>[2x]PYTVVYFPVRGRCAALRMLLADQGQSWKEEVVTVETWQEGSLKASCLYGQLPKFQDGDLTLYQSNTILRHLGRTLGLYGKDQQEAALVDMVNDGVE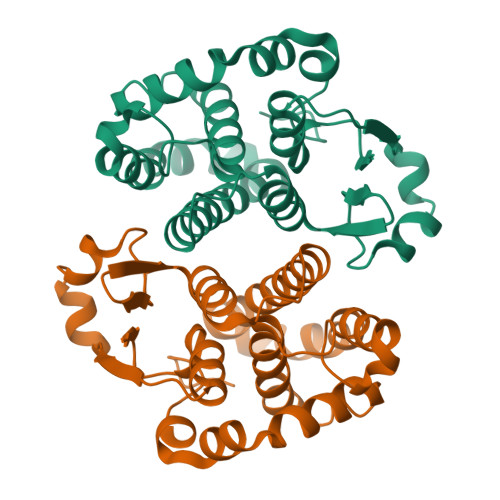DLRCKYISLIYTNYEAGKDDYVKALPGQLKPFETLLSQNQGGKTFIVGDQIAFADYNLLDLLLIHEVLAPGCLDAFPLLSAYVGRLSARPKLKAFLASPEYVNLPINGNGKQ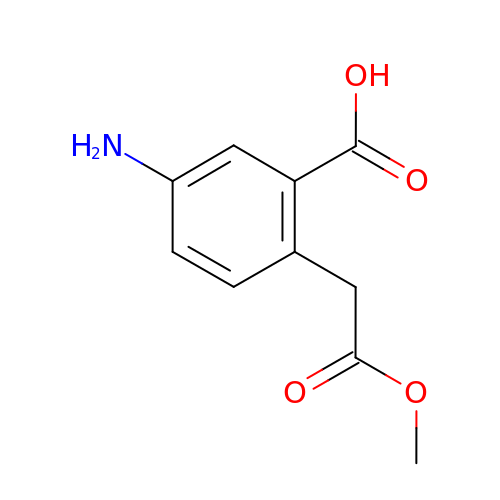5-AMINO-2-(2-METHOXY-2-OXOETHYL)BENZOIC ACID | C10 H11 N O4 | NRWKEWXVSUGTJF-UHFFFAOYSA-N> SVSEIRKAQRAEGPATILAIGTANPANCVEQSTYPDFYFKITNSEHKTELKEKFQRMCDKSMIKRRYMYLTEEILKENPNVCEYMAPSLDARQDMVVVEVPRLGKEAAVKAIKEWGQPKSKITHLIVCTTSGVDMPGADYQLTKLLGLRPYVKRYMMYQQGCFAGGTVLRLAKDLAENNKGARVLVVCSEVTAVTFRGPSDTHLDSLVGQALFGDGAAALIVGSDPVPEIEKPIFEMVWTAQTIAPDSEGAIDGHLREAGLTFHLLKDVPG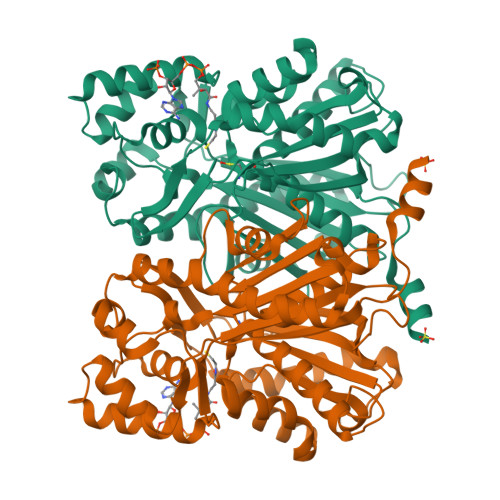IVSKNITKALVEAFEPLGISDYNSIFWIAHPGGPAILDQVEQKLALKPEKMNATREVLSEYGAMSSACVLFILDEMRKKSTQNGLKTTGEGLEWGVLFGFGPGLTIETVVLRSVAI>[4x]SNMEELTGEEVASLHSEYVMQSWHKQGGPVKPIKKADGIYFWDYDGKRYTDMSSLLVCSNLGHELPEIVDAIKEQADNMCFMAPAYASEPKSRLAKMLVDVADPDFYQRVFFTNGGADSNENAIKMARMVTGRPKIFSCYRSYHGSTIGASNASGDWRRFATELGGSAPGFVHFMNPNMYEDGYTRGVDDATVTADYLHRLDEQLQYEGPDSVAAILMESIVGANGVIL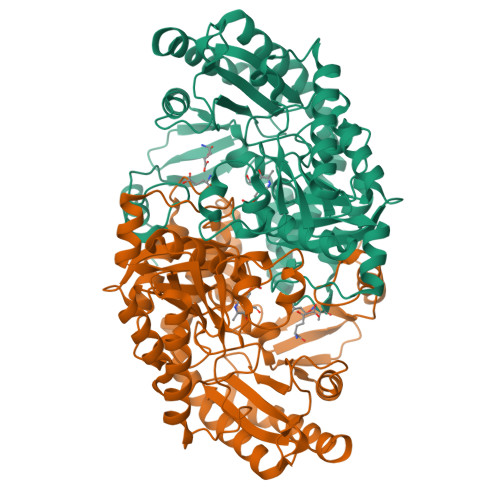PPEGYMEGVRALCDKYGILMICDEVMAGFGRTGKMFAWQNFDVKPDMFTFAKGVTCGYVPLGGVVVSKRISDYFTDHVLQCGLTYSGHTLACAAGVAAVNYYLEHDVCAHVKEMEGILKPFLESMVEKHKCVGEARCIGLFSALTIVKNKETRELMAPYHTPNSVMPQIMAKLMDLGFSTFGRETNINICPPLIITAEQLEEELPKLDKVLTWVDENLCD> TKERTFLMVKPDGVQRNLVGEVVKRFESKGLKLAGAKLMVISKDGAAAHYAELGGGPFFGG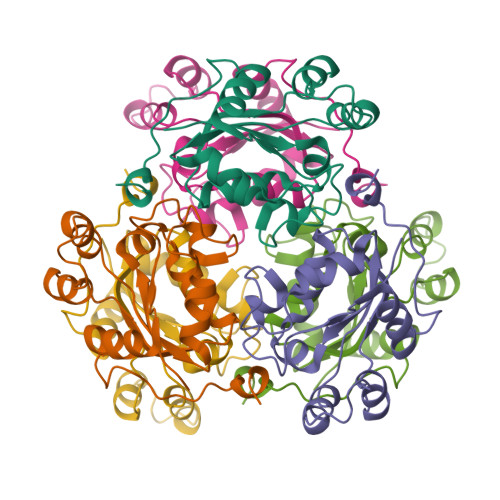LVGGATSGPVFAMVWEGLNAAATARQILGATNPSDAAPGTIRGDFGVSAGRNAIHGSDSAGSAAKEIGAFFGGGEAASGTPAAAADIYG>MIIVSGQLLRPQDIENWQIDQDLNPLLKEMIETPVQFDYHSIAELMFELKLRMNIVAAAKTLHKSGAKFATFLKTYGNTTYWRVSPEGALELKYRMPPSKAIRDIAENGPFYA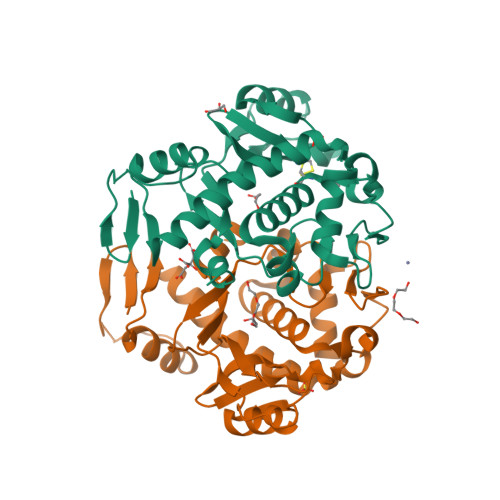FECATAIVIIYYLALIDTIGEDKFNASFDRIILYDWHYEKLPIYTETGHHFFLGDCLYFKNPEFDPQKAQWRGENVILLGEDKYFAHGLGILNGKQIIDKLNSFRKKGALQSAYLLSQATRLDVPSLFRIVRVDKLAAALEHHHHHH[2x]>GARASVLSGGELDKWEKIRLRPGGKKQYKLKHIVWASRELERFAVNPGLLETSEGCRQILGQLQPSLQTGSEELRSLYNTIAVLYCVHQRIDVKDTKEALDKIEEEQNKSKKKAQQAAADTGNNSQVSQNY[12x];>FLGKIWPS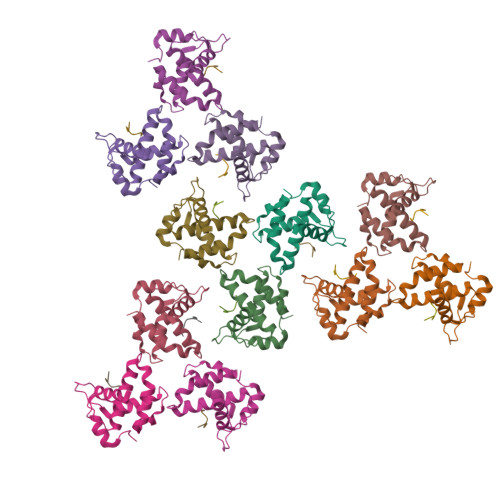HKGRPGNF[12x]>[2x]AFELPALPYAHDALASLGMSKETLEYHHDLHHKAYVDNGNKLIAGTEWEGKSVEEIVKGTYCAGAVAQSGI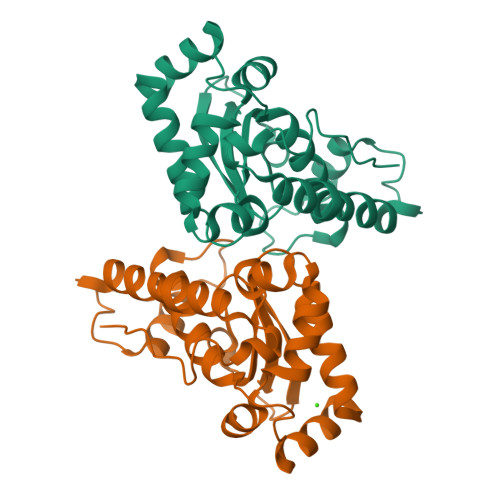FNNASQHWNHAQFWEMMGPGEDKKMPGALEKALVESFGSVAKFKEDFAAAGAGQFGSGWAWLVKDSDGALKITKTENGVNPLCFGQTALLGCDVWEHSYYIDFRNKRPAYLTNFLDKLVNWENVASRM> MIDKSAFVHPTAIVEEGASIGANAHIGPFCIVGPHVEIGEGTVLKSHVVVNGHTKIGRDNEIYQFASIGEVNQDLK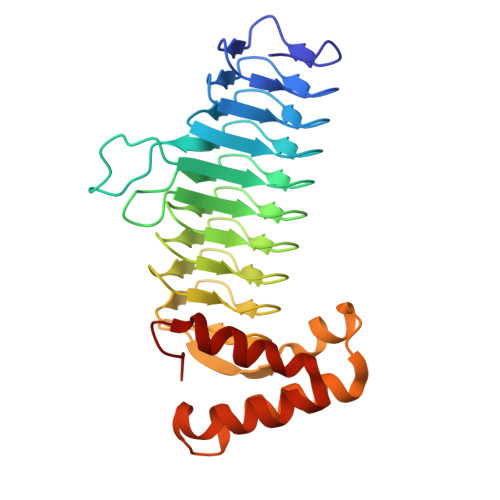YAGEPTRVEIGDRNRIRESVTIHRGTVQGGGLTKVGSDNLLMINAHIAHDCTVGNRCILANNATLAGHVSVDDFAIIGGMTAVHQFCIIGAHVMVGGCSGVAQDVPPYVIAQGNHATPFGVNIEGLKRRGFSREAITAIRNAYKLIYRSGKTLDEVKPEIAELAETYPEVKAFTDFFARSTRGLIR> DPPATVYRYDSRPPEDVFQNGFTAWGNNDNVLEHLT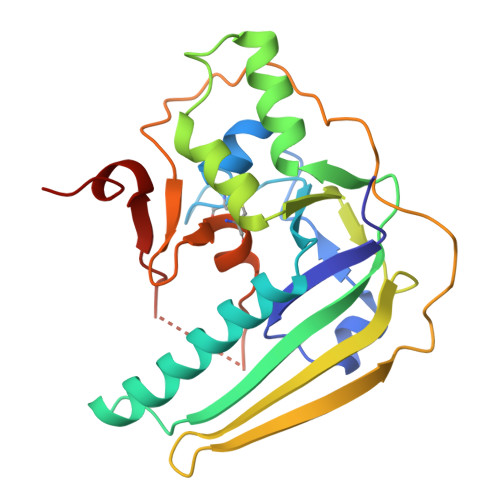GRSCQVGSSNSAFVSTSSSRRYTEVYLEHRMQEAVEAERAGRGTGHFIGYIYEVRADNNFYGAASSYFEYVDTYGDNAGRILAGALATYQSEYLAHRRIPPENIRRVTRVYHNGITGETTTTEYSNARYVSQQTRANPNPYTSRRSVASIVGTLVRMAPVVGACMARQAESSEAMAAWSERAGEAMVLVYYESIAYSF methyl 3-[[(2~{R},4~{a}~{S},6~{a}~{R},6~{a}~{S},14~{a}~{S},14~{b}~{R})-2,4~{a},6~{a},6~{a},9,14~{a}-hexamethyl-10-oxidanyl-11-oxidanylidene-1,3,4,5,6,13,14,14~{b}-octahydropicen-2-yl]carbamoylamino]oxetane-3-carboxylate 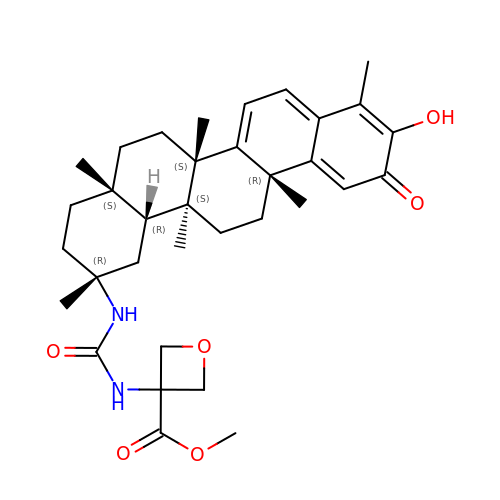| C34 H46 N2 O6 | DSRGJYYWXNYGJM-MRZDQBBQSA-N>SEPIRVLVTGAAGQIAYSLLYSIGNGSVFGKDQPIILVLLDITPMMGVLDGVLMELQDCALPLLKDVIATDKEEIAFKDLDVAILVGSMPRRDGMERKDLLKANVKIFKCQGAALDKYAKKSVKVIVVGNPANTNCLTASKSAPSIPKENFSCLTRLDHNRAKAQIALKLGVTSDDVKNVIIWGNHSSTQYPDVNHAKVKLQAKEVGVYEAVKDDSWLKGEFITTVQQRGAAVIKARKLSSAMSAAKAICDHVRDIWFGTPEGEFVSMGIISDGNSYGVPDDLLYSFPVTIKDKTWKIVEGLPINDFSREKMDLTAKELAEEKETAFEFLSSA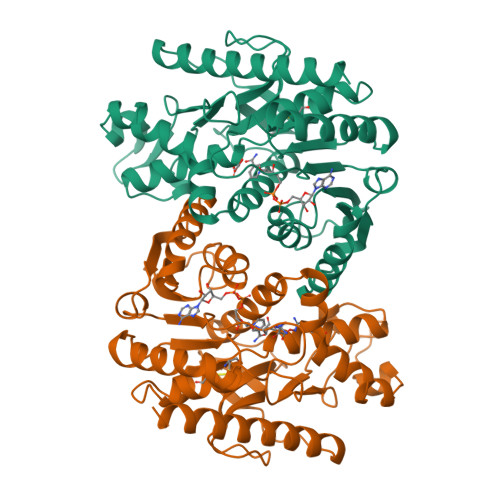[2x]> TGMDSTSTIANKIEEYLGAKSDDSKIDELLKADPSEVEYYRSGGDGDYLKNNICKITVNHSDSGKYDPCEKKLPPYDDNDQWKCQQNSSDGSGKPENICVPPRRERLCTYNLENLKFDKIRDNNAFLADVLLTARNEGEKIVQNHPDTNSSNVCNALERSFADLADIIRGTDQWKGTNSNLEKNLKQMFAKIRENDKVLQDKYPKDQKYTKLREAWWNANRQKVWEVITCGARSNDLLIKRGWRTSGKSDRKKNFELCRKCGHYEKEVPTKLDYVPQFLRWLTEWIEDFYREKQNLIDDMERHREECTREDHKSKEGTSYCSTCKDKCKKYCECVKKWKTEWENQENKYKDLYEQNKNKTSQKNTSRYDDYVKDFFEKLEANYSSLENYIKGDPYFAEYATKLSFILNPSDANNPSGETANHNDEACNCNESGISSVGQAQTSGPSSNKTCITHSSIKTNKKKECKDVKLGVRENDKDLKICVIEDTSLSGVDNCCCQDLLGILQENCSDNKRGSSSNDSCDNKNQDECQKKLEKVFASLTNGYKCDKCKSGTSRSKKKWIWKKSSGNEEGLQEEYANTIGLPPRTQSLYLGNLPKLENVCEDVKDINFDTKEKFLAGCLIVSFHEGKNLKKRYPQNKNSGNKENLCKALEYSFADYGDLIKGTSIWDNEYTKDLELNLQNNFGKLFGKYIKKNNTAEQDTSYSSLDELRESWWNTNKKYIWTAMKHGAEMNITTCNADGSVTGSGSSCDDIPTIDLIPQYLRFLQEWVENFCEQRQAKVKDVITNCKSCKESGNKCKTECKTKCKDECEKYKKFIEACGTAGGGIGTAGSPWSKRWDQIYKRYSKHIEDAKRNRKAGTKNCGTSSTTNAAASTDENKCVQSDIDSFFKHLIDIGLTTPSSYLSNVLDDNICGADKAPWTTYTTYTTTEKCNKERDK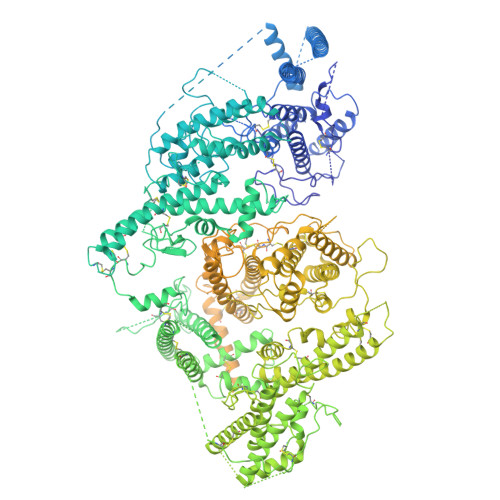SKSQSSDTLVVVNVPSPLGNTPYRYKYACQCKIPTNEETCDDRKEYMNQWSCGSARTMKRGYKNDNYELCKYNGVDVKPTTVRSNSSKLDGNDVTFFNLFEQWNKEIQYQIEQYMTNANISCIDEKEVLDSVSDEGTPKVRGGYEDGRNNNTDQGTNCKEKCKCYKLWIEKINDQWGKQKDNYNKFRSKQIYDANKGSQNKKVVSLSNFLFFSCWEEYIQKYFNGDWSKIKNIGSDTFEFLIKKCGNNSAHGEEIFNEKLKNAEKKCKENESTDTNINKSETSCDLNATNYIRGCQSKTYDGKIFPGKGGEKQWICKDTIIHGDTNGACIPPRTQNLCVGELWDKSYGGRSNIKNDTKELLKEKIKNAIHKETELLYEYHDTGTAIISKNDKKGQKGKNDPNGLPKGFCHAVQRSFIDYKNMILGTSVNIYEHIGKLQEDIKKIIEKGTPQQKDKIGGVGSSTENVNAWWKGIEREMWDAVRCAITKINKKNNNSIFNGDECGVSPPTGNDEDQSVSWFKEWGEQFCIERLRYEQNIREACTINGKNEKKCINSKSGQGDKIQGACKRKCEKYKKYISEKKQEWDKQKTKYENKYVGKSASDLLKENYPECISANFDFIFNDNIEYKTYYPYGDYSSICSCEQVKYYKYNNAEKKNNKSLCYEKDNDMTWSKKYIKKLENGRSLEGVYVPPRRQQLCLYELFPIIIKNEEGMEKAKEELLETLQIVAEREAYYLWKQYNPTGKGIDDANKKACCAIRGSFYDLEDIIKGNDLVHDEYTKYIDSKLNEIFGSSDTNDIDTKRARTDWWENETITNGTDRKTIRQLVWDAMQSGVRYAVEEKNENFPLCMGVEHIGIAKPQFIRWLEEWTNEFCEKYTKYFEDMKSKCDPPKRADTCGDNSNIECKKACANYTNWLNPKRIEWNGMSNYYNKIYRKSNKESEGGKDYSMIMAPTVIDYLNKRCHGEINGNYICCSCKNIGAYNTTSGTVNKKLQKKETECEEEKGPLDLMNEVLNKMDKKYSAHKMKCTEVYLEHVEEQLNEIDNAIKDYKLYPLDRCFDDQTKMKVCDLIADAIGCKDKTKLDELDEWNDMDLRGTYNKHKGVLIPPRRRQLCFSRIVRGPANLRSLNEFKEEILKGAQSEGKFLGNYYKEHKDKEKALEAMKNSFYDYEDIIKGTDMLTNIEFKDIKIKLDRLLEKETNNTKKAEDWWKTNKKSIWNAMLCGYKKSGNKIIDPSWCTIPTTETPPQFLRWIKEWGTNVCIQKQEHKEYVKSKCSNVTNLGAQASESNNCTSEIKKYQEWSRKRSIRWETISKRYKKYKRMDILKDVKEPDANTYLREHCSKCPCGFNDMEEMNNNEDNEKEAFKQIKEQVKIPAELEDVIYRIKHHEYDKGNDYICNKYKNIHDRMKKNNGNFVTDNFVKKSWEISNGVLIPPRRKNLFLYIDPSKICEYKKDPKLFKDFIYWSAFTEVERLKKAYGGARAKVVHAMKYSFTDIGSIIKGDDMMEKNSSDKIGKILGDTDGQNEKRKKWWDMNKYHIWESMLCGYREAEGDTETNENCRFPDIESVPQFLRWFQEWSENFCDRRQKLYDKLNSECISAECTNGSVDNSKCTHACVNYKNYILTKKTEYEIQTNKYDNEFKNKNSNDKDAPDYLKEKCNDNKCECLNKHIDDKNKTWKNPYETLEDTFKSKCDCPKPLPSPIKPDDLPPQADEPFGTKHHHHHH>GMFHRRKRPYNTRNYGHDDKKFKSQYIDIMPDFSPSGLLELESNNKEGIALKHVEP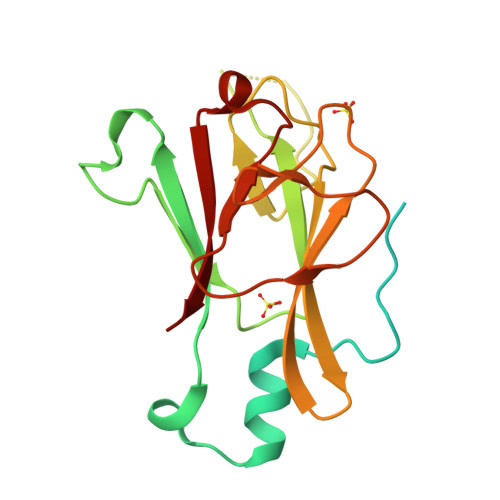QDAISPDNYMDMLGLEARDRTMYELVIYRKNDKDKGPWKRYDLNGRSCYLVGRELGHSLDTDLDDRTEIVVADIGIPEETSSKQHCVIQFRNVRGILKCYVMDLDSSNGTCLNNVVIPGARYIELRSGDVLTLSEFEEDNDYELIFMNV[2x]> MEVLKLQ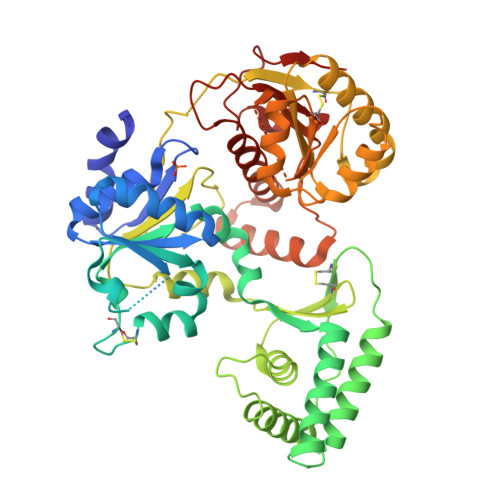LRQWQAEKLGEAINALKHGKTLLLNAKPGLGKTVFVEVLGMQLKKKVLIFTRTHSQLDSIYKNAKLLGLKTGFLIGKSASCIYAQGDEEPDEINCSKCRLKDKIKTIEDKEPSKLIEEFKDAVDYCPYYSLRANLKDKDVIAMTYPYLFQKPIRNSVFCNKDDCLKLEDYLIVIDEAHNLLEADKWFTRKISRKMLERALKEIEIVERLNRIDAKKVKDYINLLIDYMSKLIKDGRCHELSLMPLPDRETNGELIVVTRAYLNIDEGPVKKSSLKSLLKFVEMKGDLYNCNGSLVKVPSDVNQLIEDALNVKTFKVLMSGTLPESLTLTNSYKIVVNESYGRGEYYYCPNVTSELRKRNSNIPIYSILLKRIYENSSKSVLVFFPSYEMLESVRIHLSGIPVIEENKKTRHEEVLELMKTGKYLVMLVMRAKESEGVEFREKENLFESLVLAGLPYPNVSDDMVRKRIERLSKLTGKDEDSIIHDLTAIVIKQTIGRAFRDPNDYVKIYLCDSRYREYFADLGISEKEIKLFA> MQAGPAMERHYYTYLIKEEFANHYFGRESVMFELFQDYHWTSLEKQQYEMTEKQIQYITQPIPILHMHQRLKMNLNKTDYR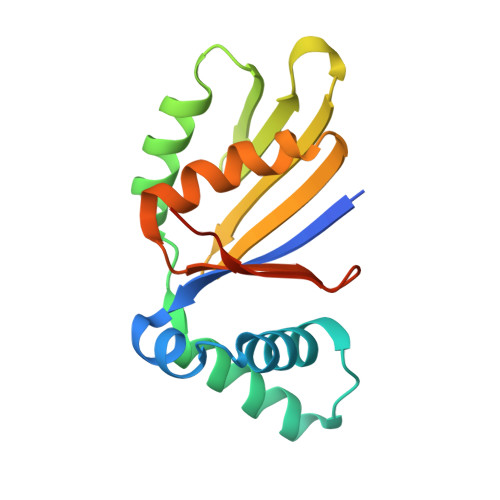QLDYIYRIALPKAKGHATFMMKEHMIEIVASGDYEAETIFFEVLRKVSPCFLAMDFNSKRYGWLNPVKERNFV>XGEIAALKQEIAALKK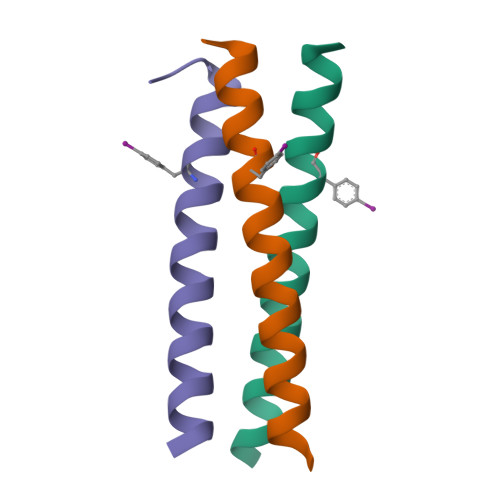EIAALKFEIAALKQGYY[3x]>GEEKGSSEDAKTIKVAASATPHAEILEQAKSILKKEGYQLEVTVFDDYVQPNEVVESGEFDANYFQHVPYLESFNEEKGTH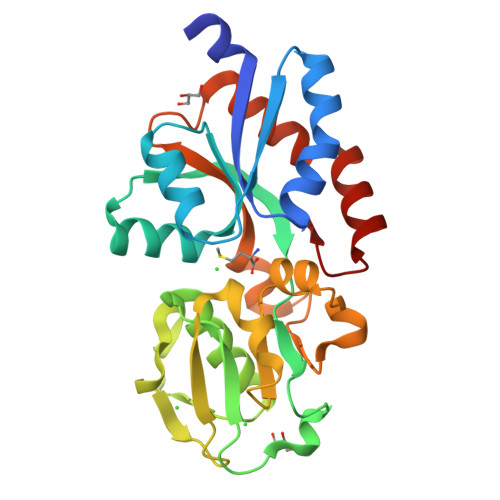LVDAGDIHYEPFGIYPGTKKSLDEISEGDKIAVPNDTTNEARALLLLQDNGIITLKDGAGLNATVNDIEENPYNVEIVELEAAQVARVTGETAYVVLNGNYALEAGYSVAKDALAYEKSDSEAAKTYVNIIAVKEGNEKEEKIQALVKALKSDEIKEYIEKTYDGAVIPFE[2x]(2E)-2-[({3-hydroxy-2-methyl-5-[(phosphonooxy)methyl]pyridin-4-yl}methyl)imino]-3-[(2-hydroxyphenyl)amino]propanoic 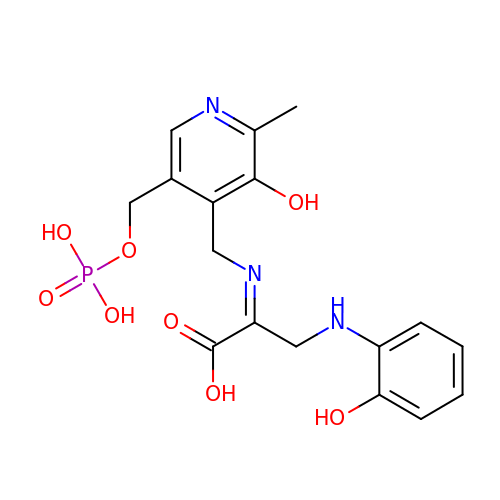acid | C17 H20 N3 O8 P | MKNJFLJOSVXALN-XMHGGMMESA-N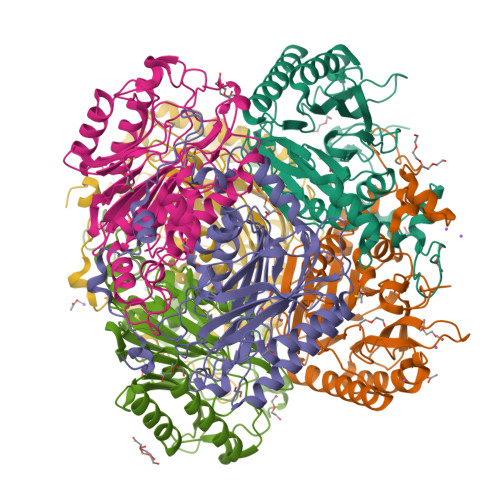>[6x]MGSSGSMVKPISGFLTALIQYPVPVVESRADIDKQIQQIIKTIHSTKSGYPGLELIVFPEYSTQGLNTKKWTTEEFLCTVPGPETDLFAEACKESKVYGVFSIMEKNPDGGEPYNTAVIIDPQGEMILKYRKLNPWVPVEPWKAGDLGLPVCDGPGGSKLAVCICHDGMFPEVAREAAYKGANVLIRISGYSTQVSEQWMLTNRSNAWQNLMYTLSVNLAGYDGVFYYFGEGQVCNFDGTTLVQGHRNPWEIVTAEVYPELADQARLGWGLENNIYNLGSRGYVATPGGVKENPYTFVKDLAEGKYKVPWEDEIKVKDGSIYGYPVKKTIHSWFRVDPLEHHHHHH> MGHHHHHHENLYFQGHMASGSLSENVLFGMGNPLLDISAVVDKDFLDKYSLKPNDQILAEDKHKELFDELVKKFKVEYHAGGSTQNSMKVAQWLIQEPHKAATFFGCIGIDKFGEILKRKAADAHV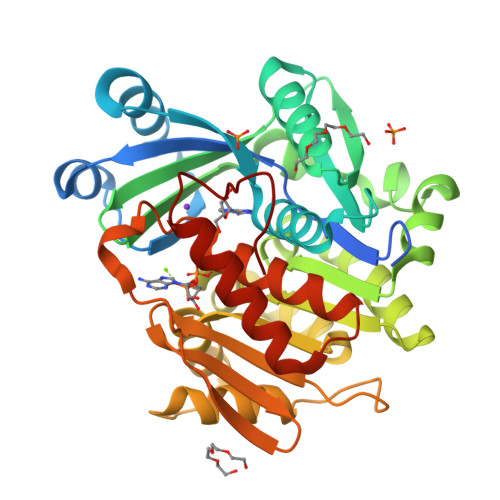DAHYYEQNEQPTGTCAACITGGNRSLVANLAAANCYKKEKHLDLERNWVLVEKARVYYIAGFFLTVSPESVLKVARYAAENNRVFTLNLSAPFISQFFKEALMDVMPYVDILFGNETEAATFAREQGFETKDIKEIAKKAQALPKVNSKRQRTVIFTQGRDDTIVAAENDVTAFPVLDQNQEEIIDTNGAGDAFVGGFLSQLVSDKPLTECIRAGHYAASVIIRRTGCTFPEKPDFH> DCPSGWSSYEGHCYKPFNEPKNWADAERFCKLQPKHSHL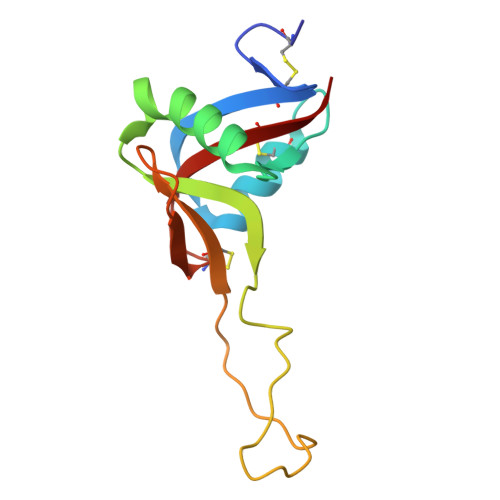VSFQSAEEADFVVKLTRPRLKANLVWMGLSNIWHGCNWQWSDGARLNYKDWQEQSECLAFRGVHTEWLNMDCSSTCSFVCKFKA>[3x]GPKVPEFGSSRISALEYATTRKKSEVVYSGVSVTIPTAPTNLVSLLKTLTPSSGTLAPFFDTVNNKMVVFNENKTLFFKLSIVGTWPSGTANRSMQ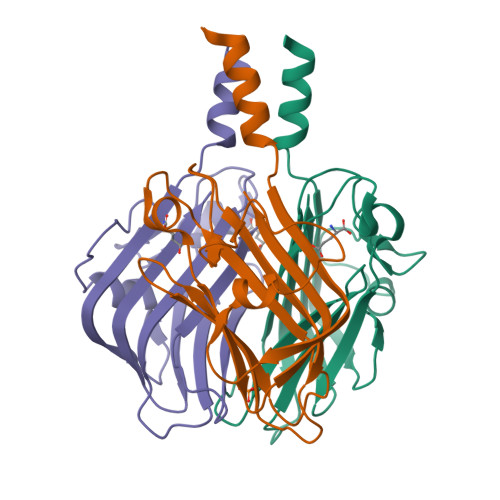LTFSGSVPDTLVSSRNSATTTDNILLATFFSVDKDGFLATNGSTLTIQSNGAAFTATTIKIIAEQ> GMVPISPIETVPVKLKPGMDGPKVKQWPLTEEKIKALVEICTEMEKEGKISKIGPENPYNTPVFAIKKKDSTKWRKLVDFRELNKRTQDFWEVQLGIPHPAGLKKKKSVTVLDVGDAYFSVPLDEDFRKYTAFTIPSINNETPGIRYQYNVLPQGWKGSPAIFQSSMTKILEPFAAQNPDIVIYQYMDDLYVGSDLEIGQHRTKIEELRQHLLRWGLTTPDKKHQKEPPFLWMGYELHPDKWTVQPIVLPEKDSWTVNDIQKLVGKLNWASQIYPGIKVRQLSKLLRGTKALTEVIPLTEEAELELAENREILKEPVHGVYYDPSKDLIAEIQKQGQGQWTYQIYQEPFKNLKTGKYARMRGAHTNDVKQLTEAVQKITTESIVIWGKTPKFKLPIQKETWETWWTEYWQATWIPEWEFVNTPPLVKLWYQLEKEPIVGAETFYVDGAANRETKLGKAGYVTNKGRQKVVPLTNTTNQKTELQAIYLALQDSGLEVNIVTDSQYALGIIQAQPDKSESELVNQIIEQLIKKEKVYLAWVPAHKGIGGNEQVDKLVSAG;> PISPIETVPVKLKPGMDGPKVKQWPLTEEKIKALVEICTEMEKEGKISKIGPENPYNTPVFAIKKKDSTKWRKLVDFRELNKRTQDFWEVQLGIPHPAGLKKKKSVTVLDVGDAYFSVPLDEDFRKYTAFTIPSINNETPGIRYQYNVLPQGWKGSPAIFQSSMTKILEPFKKQNPDIVIYQYMDDLYVGSDLEIGQHRTKIEELRQHLLRWGLTTPDKKHQKEPPFLWMGYELHPDKWTVQPIVLPEKDSWTVNDIQ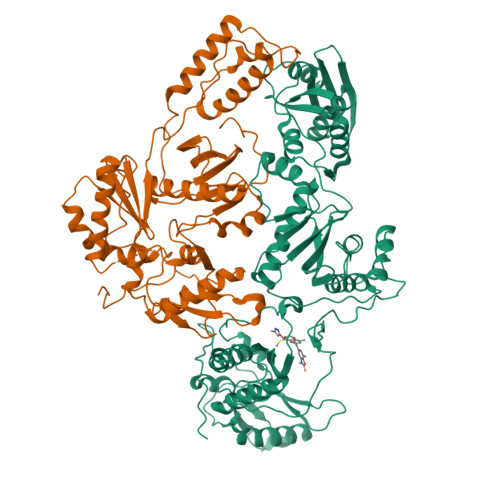KLVGKLNWASQIYPGIKVRQLSKLLRGTKALTEVIPLTEEAELELAENREILKEPVHGVYYDPSKDLIAEIQKQGQGQWTYQIYQEPFKNLKTGKYARMRGAHTNDVKQLTEAVQKITTESIVIWGKTPKFKLPIQKETWETWWTEYWQATWIPEWEFVNTPPLVKLWYQ> MFNRTTQLKSKHPCSVCTRRKVKCDRMIPCGNCRKRGQDSECMKSTKLITASSSKEYLPDLLLFWQNYEYWITNIGLYKTKQRDLTRTPANLDTDTEECMFWMNYLQKDQSFQLMNFAMENLGALYFGSIGDISELYLRVEQYWDRRADKNHSVDGKYWDALIWSVFTMCIYYMPVEKLAEIFSVYPLHEYLGSNKRLNWEDGMQLVMCQNFARCSLFQLKQCDFMAHPDIRLVQAYLILATTTFPYDEPLLANSLLTQCIHTFKNFHVDDFRPLLNDDPVESIAKVTLGRIFYRLCGCDYLQSGPRKPIALHTEVSSLLQHAAYLQDLPNVDVYREENSTEVLYW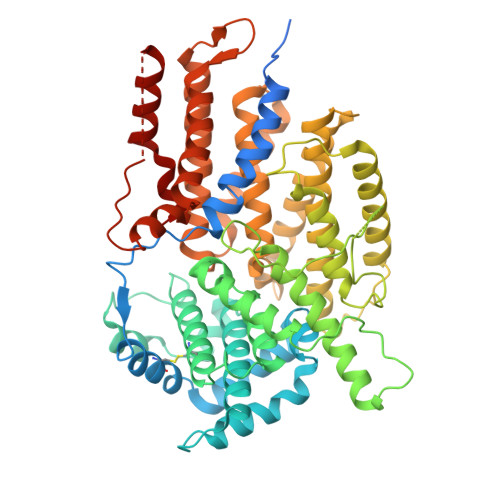KIISLDRDLDQYLNKSSKPPLKTLDAIRRELDIFQYKVDSLEEDFRSNNSRFQKFIALFQISTVSWKLFKMYLIYYDTADSLLKVIHYSKVIISLIVNNFHAKSEFFNRHPMVMQTITRVVSFISFYQIFVESAAVKQLLVDLTELTANLPTIFGSKLDKLVYLTERLSKLKLLWDKVQLLDSGDSFYHPVFKILQNDIKIIELKNDEMFSLIKGLGSLVPLNKLRQESLLEEEDENNTEPSDFRTIVEEFQSEYNISDILS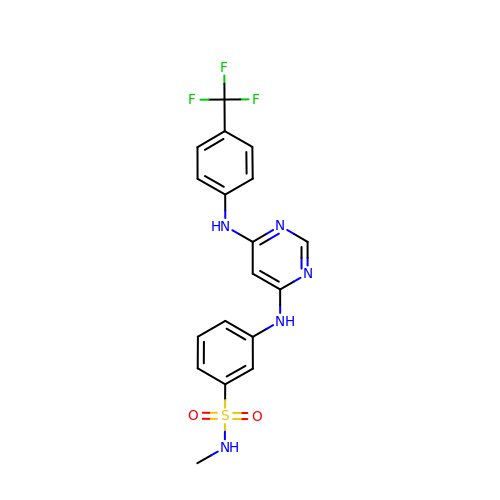N-methyl-3-[(6-{[4-(trifluoromethyl)phenyl]amino}pyrimidin-4-yl)amino]benzene-1-sulfonamide | C18 H16 F3 N5 O2 S | UNIMPGVNGHKXEY-UHFFFAOYSA-N>[6x]EAISYSMPEETESGYLVANLAQDLGLRVGELTTRGARIHHNGNKELLQLDAERGNLLLKEKPDREALCGATEPCVLHFQIILENPVQFFQTDLQFTDINDHFPEFPDTEMLLKIQEIAQPGTVFPLKAAQDPDIGSNAVQNYTVSPNLHFHVVTLSRSDDRKYPELVLDRALDREEQPELTLILTALDGGAPPKSGTTT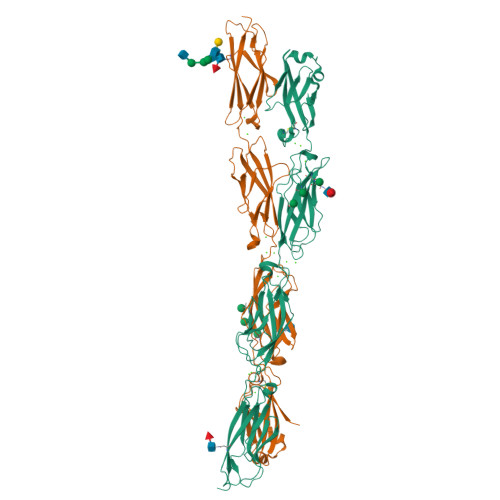VRIEVVDINDNAPQFLQSLYAVEVPENSPLNALVVTVSARDLDAGIHGNVAYSLFQGGGGPQPFVIDEITGEIRLKGALDFEATSYYTMEIVATDSGGLSGKCTVAIQVLDVNDNAPKLTISSLTSSIPENAPEAVVAVFSVSDPDSGDNGRMVCSIQNGLPFLLKPTFKNFYTLVTERPLDRESNAEYNITITVSDLGTPRLTTQHTITVQVSDINDNHHHHHHHH> MEYAARRNQKGAFEGFYKLIMRRNSVYV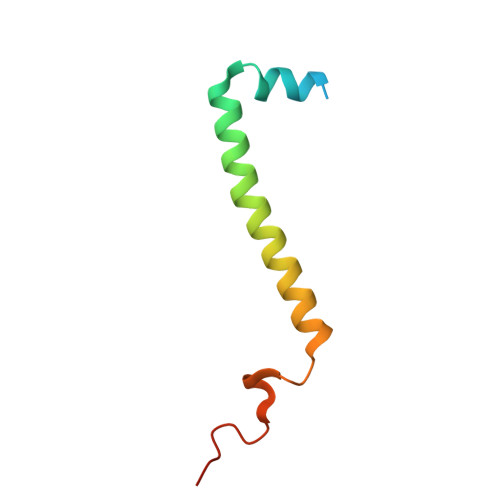TFIIAGAFFGERAVDYGVHKLWERNNVGKRYEDISVLGQRPVEE>[2x]GMADIDQASKTEMEAAAFRHLLRHLDEHKDVQNIDLMIQADF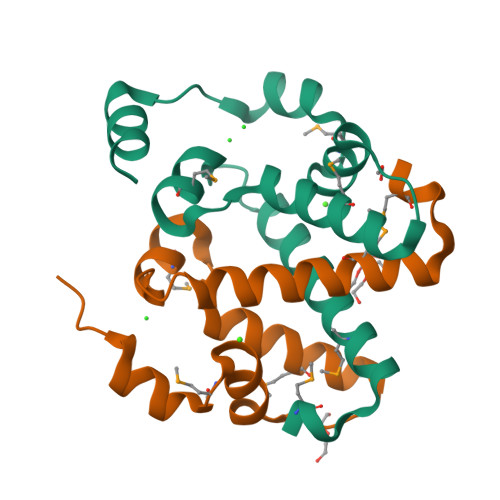CRNCLAKWLMEAATEQGVELDYDGAREYVYGMPFAEWKTLYQKPASEAQLAAFEAKQAARKR> MHHHHHHKLITLLLRSSKSEDLRLSIPVDFTVKDLIKRYCTEVKISFHERIRLEFEGEWLDPNDQVQSTELEDEDQVSVVLD;> MHHHHHHSSLCKTRLQEERKQWRRDHPFGFYAKPCKSSDGGLDLMNWKVGIPGKPKTSWEGGLYKLTMAFPEEYPT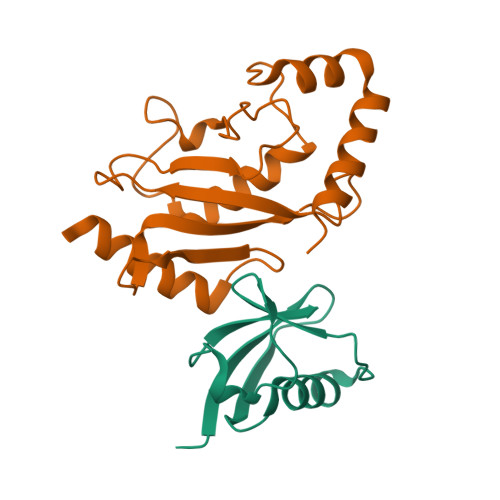RPPKCRFTPPLFHPNVYPSGTVCLSILNEEEGWKPAITIKQILLGIQDLLDDPNIASPAQTEAYTMFKKDKVEYEKRVRAQARENAP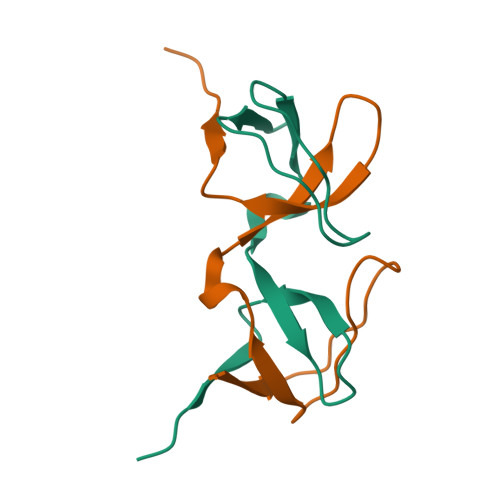>[2x]KKYAKSKYDFVARNSSELSVMKDDVLEILDDRRQWWKVRNASGDSGFVPNNILDIMRTPE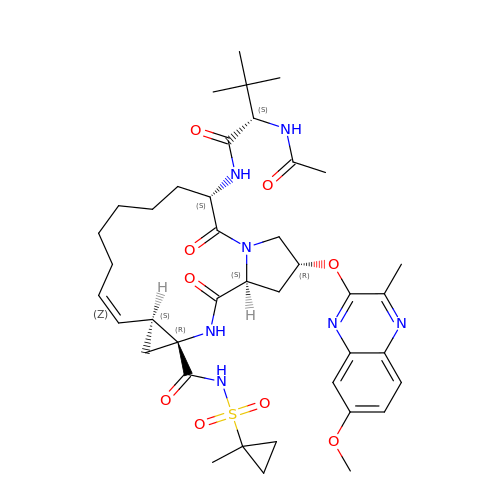(2R,6S,12Z,13aS,14aR,16aS)-6-[(N-acetyl-3-methyl-L-valyl)amino]-2-[(7-methoxy-3-methylquinoxalin-2-yl)oxy]-N-[(1-methylcyclopropyl)sulfonyl]-5,16-dioxo-1,2,3,6,7,8,9,10,11,13a,14,15,16,16a-tetradecahydrocyclopropa[e]pyrrolo[1,2-a][1,4]diazacyclopentadecine-14a(5H)-carboxamide | C40 H55 N7 O9 S | YOHPIODWEANJQZ-UYLSUIKTSA-N5-(HYDRO)PEROXOISOURATE | C5 H4 N4 O5 | 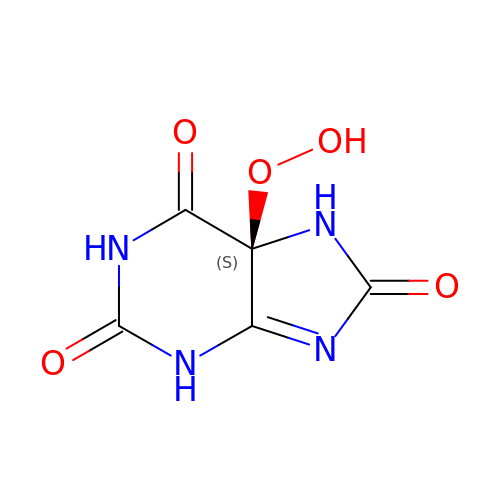XHKXPKDICPOLRC-YFKPBYRVSA-N>[16x]XGEIAQALKEIA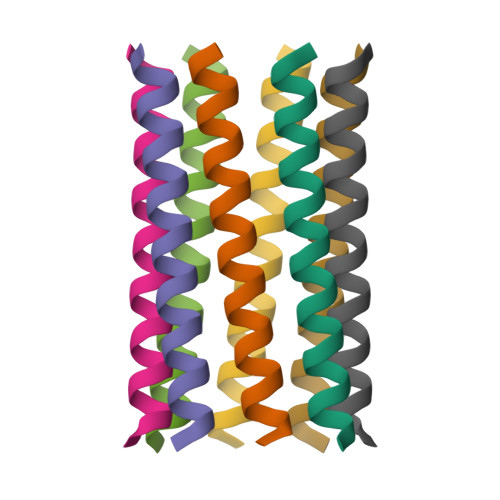KALKEIAWAKKEIAQALKGX>[4x]RVDDPAGKAAQYHKEYALFRSANMPSPDKLATGVGFHSFRIPAVVRTNTGRILAFAEGRRHNNRDYGDINLVYKRTKSPTNNGENPTDWESLREVVGTGPHTWGNPTPVVDGNTIYLFLSMNDGAYSQNGGNTLPDGTKTKKIDSTWVGRRHLYLTTSTDDGDTWTKPVDMTKTLTPDGQAWDAVGPGNG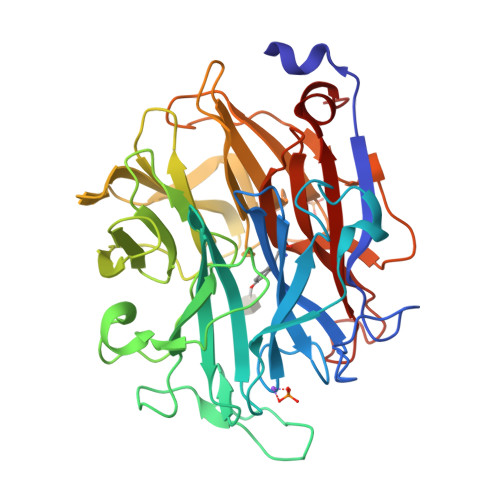IKLSTGELVIPAQGRNIIGRGPSGNRTWSMQILKGAGSEGTICQTPDGKLMRNDRPGPMGHRSVARGTLAGLGPFATDNGLPDPACQGSILSYNSDEPARTIFMNSASTDRRTAMRVRISYDKDAAKFNFGRELKDAPLGNVGNEGGYSSMTKTSDYKIGALVESDWYEDKGGEKSHRCIIWRRFNLSWIINGPNN> MRGSHHHHHHGSPSQTSFKPLTVVDGVAVNMPNNHPDLSNWLPSIELCVKKYNEKHTGGLKPIEVIATGGQNNQLT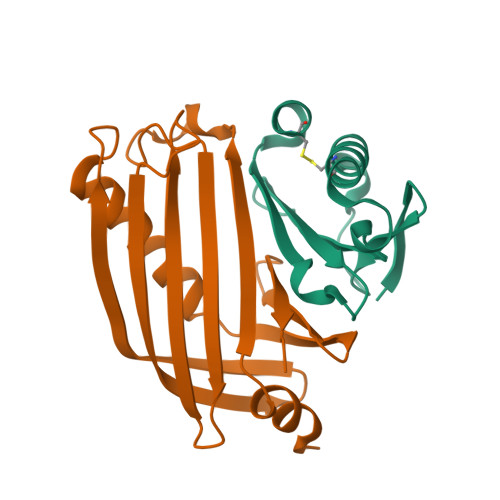LNYIHSPEVSGENITLRIVANPNDAIKVCE;> MGSSHHHHHHSQDPNSDFKLEQVLTSREWQSKMVSLIKTNSNRPAMGPLSRVDVTSNVKYLPNGTYLRVSIVKLFSDDNSAESVINISEFGEWDISDNYLLVTPVEFKDISSNQSKDFTDEQLQLITQLFKMDAQQSRRVDIVNERTILFTSLSHGSTVLFSNS>[3x]ENLMQVYQQARLSNPE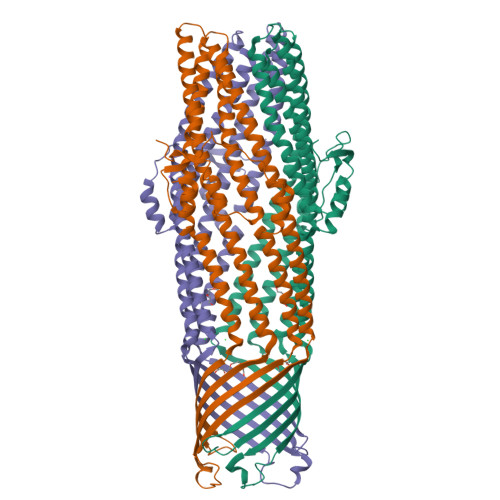LRKSAADRDAAFEKINEARSPLLPQLGLGADYTYSNGYRDANGINSNATSASLQLTQSIFDMSKWRALTLQEKAAGIQDVTYQTDQQTLILNTATAYFNVLNAIDVLSYTQAQKEAIYRQLDQTTQRFNVGLVAITDVQNARAQYDTVLANELTARNNLDNAVEQLRQITGNYYPELAALNVENFKTDKPQPVNALLKEAEKRNLSLLQARLSQDLAREQIRQAQDGHLPTLDLTASTGISDTSYSGSKTRGAAGTQYDDSNMGQNKVGLSFSLPIYQGGMVNSQVKQAQYNFVGASEQLESAHRSVVQTVRSSFNNINASISSINAYKQAVVSAQSSLDAMEAGYSVGTSTIVDVLDATTTLYNAKQELANARYNYLINQLNIKSALGTLNEQDLLALNNALSKPVSTNPE> MLRRSPVPRRYRTAWRELLHPLPVWARRQQWLK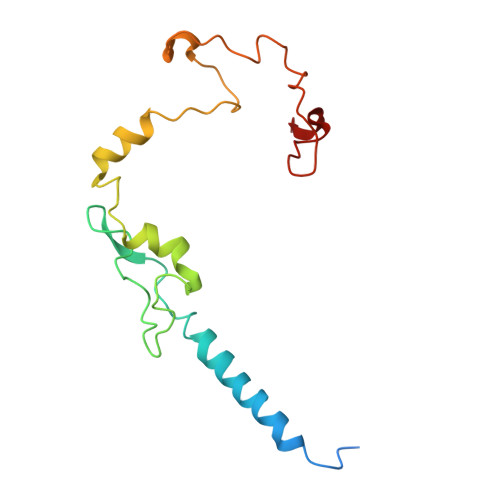RDTVEMNEAILREPYYRIKTFAQPAAFVSPRVSESAAHEPDTQQSSRYGVDRQLRGPRRAVSPERLQELREQLQFVGSIGPKVPPAAGAGTAYQDEYGTRLRPRYPQSWDTVPPHQPSRSEI>MRRLLLLCEYDGTLFAGLQRQGRGLRTVQGELERALPGIGALPKAVAAGRTDAGVHALAMPFHVDVESAIPVEKVPEALNRLLPEDLKVVGAREVAPDFHARKDALWRAYRYRILVRPHPSPLLRHRALWVRRPLDLEAMEEALSLLLGRHNFLGFAKEETRPGER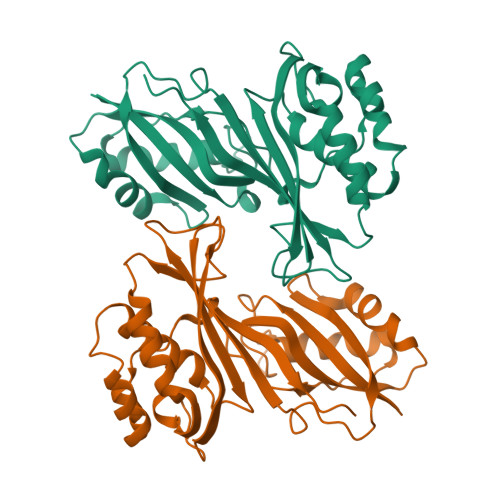ELLEARLQVAEGEAGLEVRLYFRGKSFLRGQVRGMVGTLLEVGLGKRPPESLKAILKTADRRLAGPTAPAHGLYFVEAAYPEE[2x]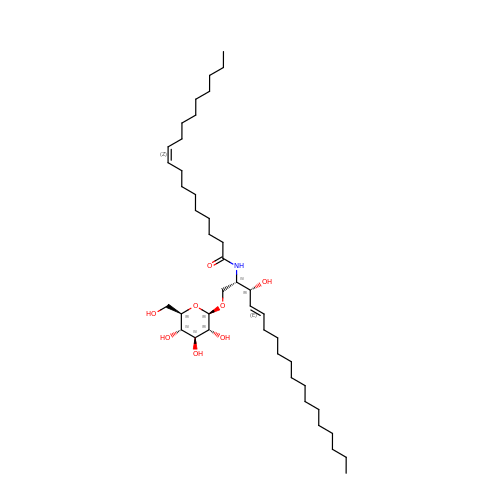(9Z)-N-[(2S,3R,4E)-1-(beta-D-glucopyranosyloxy)-3-hydroxyoctadec-4-en-2-yl]octadec-9-enamide | C42 H79 N O8 | MVGFIPNJBNBHNC-HVFXMTMESA-N> ALTEGLGDELEEVIVEKTKQTVASISSGPKHTQKVPILTANETGATMPVLPSDSIETRTTYMHFNGSETDVECFLGRAACVHVTEIQNKDATGIDNHREAKLFNDWKINLSSLVQLRKKLELFTYVRFDSEYTILATASQPDSANYSSNLVVQAMYVPPGAPNPKEW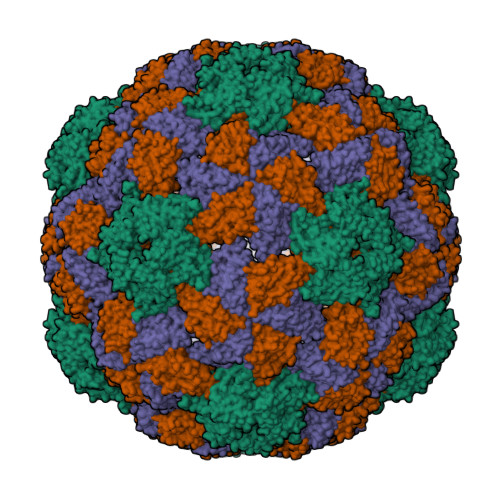DDYTWQSASNPSVFFKVGDTSRFSVPYVGLASAYNCFYDGYSHDDAETQYGITVLNHMGSMAFRIVNEHDEHKTLVKIRVYHRAKHVEAWIPRAPRALPYTSIGRTNYPKNTEPVIKKRKGDIKSY;> SPNVEACGYSDRVQQITLGNSTITTQEAANAVVCYAEWPEYLPDVDASDVNKTSKPDTSVCRFYTLDSKTWTTGSKGWCWKLPDALKDMGVFGQNMFFHSLGRSGYTVHVQCNATKFHSGCLLVVVIPEHQLASHEGGNVSVKYTFTHPGERGIDLSSANEVGGPVKDVIYNMNGTLLGNLLIFPHQFINLRTNNTATIVIPYINSVPIDSMTRHNNVSLMVIPIAPLTVPTGATPSLPITVTIAPMCTEFSGIRSKSIVPQ;> GLPTTTLPGSGQFLTTDDRQSPSALPNYEPTPRIHIPGKVHNLLEIIQVDTLIPMNNTHTKDEVNSYLIPLNANRQNEQVFGTNLFIGDGVFKTTLLGEIVQYYTHWSGSLRFSLMYTGPALSSAKLILAYTPPGARGPQDRREAMLGTHVVWDIGLQSTIVMTIPWTSGVQFRYTDPDTYTSAGFLSCWYQTSLILPPETTGQVYLLSFISACPDFKLRLMKDTQTISQTV>DTGCAVSWSGKELKCGSGIFVIDNVHTWTEQYKFQPESPARLASAILNAHEDGVCGIRSTTRLENIMWKQITNELNYVLWEGGHDLTVVAGDVKGVLSKGKRALAPPVNDLKYSWKTWGKAKIFTPEAKNSTFLIDGPDTSECPNERRAWNFLEVEDYGFGMFTTNIWMKFREGSSEVCDHRLMSAAIKDQKAVHADMGYWIESSKNQTWQIEKASLIEVKTCLWPKTHTLWSNGVLESQMLIPKAYAGPFSQHNYRQGYATQTVGPWHLGKLEIDFGECPGTTVTIQEDCDHRGPSLRTTTASGKLV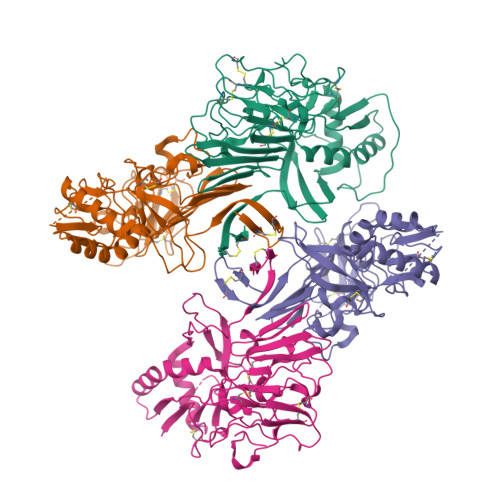TQWCCRSCTMPPLRFLGEDGCWYGMEIRPLSEKEENMVKSQVSAHHHHHH[4x]> KFFEQ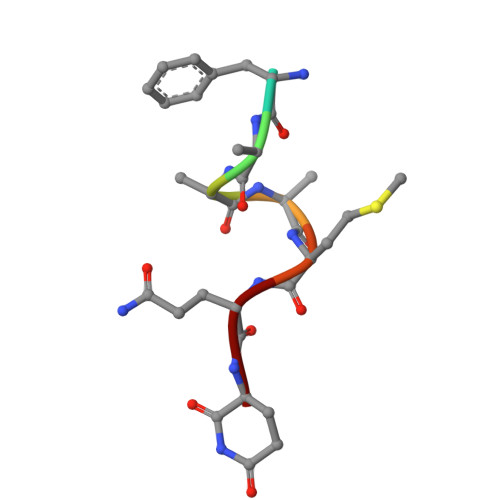MQQ>MVKIESVAIVGGGSSGWMTAAALSKLCPQLEIALIEDPNIKTVGVGESTLGHFNKFLHLLDLKDEDWMPACNATYKNSIRFTNFREGKGEVFEYPFGPSLDVSFFSQTDGINTWGKLANKYPEDFPPETFARFVNSNTYLAEHNRLTRNKDNKIPNFNFDWDTAYHIDAELFGQYLKEKIALPNGVKHIQGKVTGYQKESPNNHNFKYIILDQETAIFADLYIDCTGFKSLLLGEFMGEAFSPFSKKLANDKAMATRIPYENREEEMHNVTDCHAMKNGWVWNIPLWNRIGTGYCYSSRFVSKDDAEAEFREHLGERGKDAKIFHIDIGHGKRTRAWVNNCVGIGLSYGFIEPLESTGLLTTHENIENLVYLINQRDGYVTQAERDGFNYTCDHQIDSFSDFVAMHYAYSMRTDTPYWKWCTQMCNYMPESMGPHRQKQSTWQDLSTD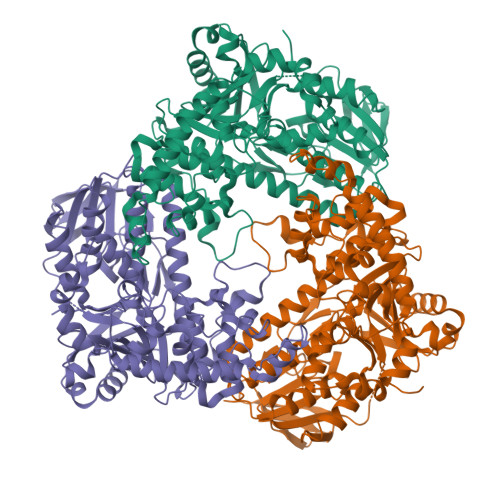TIGLNTWHINHNGISFIIAGHGLRPQSYDKLSEVLLKRNNESDYYYEDIRKDWLKHYESMVEYVKTLPTHYEFLRDEIYGSAE[6x]> MGNIMSASFAPECTDLKTKYDSCFNEWYSEKFLKGKSVEN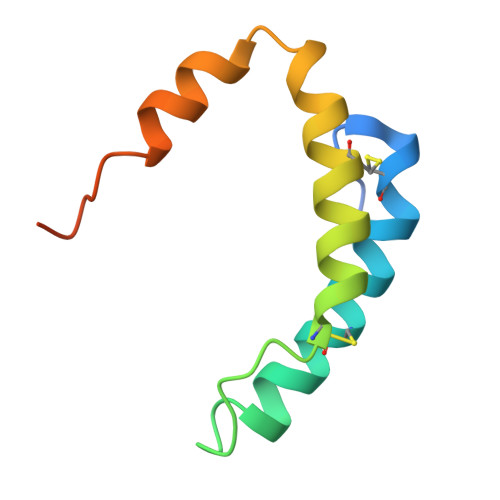ECSKQWYAYTTCVNAALVKQGIKPALDEAREEAPFENGGKLKEVDK>MGSETPQAEVGPTGCPHRSGPHSAKGSLEKGSPEDKEAKEPLWIRPDAPSRCTWQLGRPASESPHHHTAPAKSPKILPDILKKIGD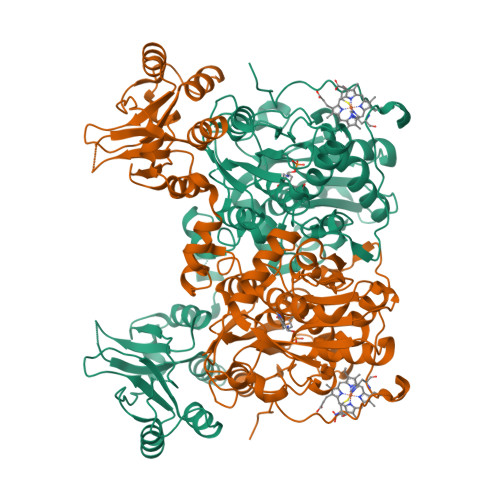TPMVRINKIGKKFGLKCELLAKCEFFNAGGSVKDRISLRMIEDAERDGTLKPGDTIIEPTSGNTGIGLALAAAVRGYRCIIVMPEKMSSEKVDVLRALGAEIVRTPTNARFDSPESHVGVAWRLKNEIPNSHILDQYRNASNPLAHYDTTADEILQQCDGKLDMLVASVGTGGTITGIARKLKEKCPGCRIIGVDPEGSILAEPEELNQTEQTTYEVEGIGYDFIPTVLDRTVVDKWFKSNDEEAFTFARMLIAQEGLLCGGSAGSTVAVAVKAAQELQEGQRCVVILPDSVRNYMTKFLSDRWMLQKGFLKEEDLTEKKPWWWHLRVQELGLSAPLTVLPTITCGHTIEILREKGFDQAPVVDEAGVILGMVTLGNMLSSLLAGKVQPSDQVGKVIYKQFKQIRLTDTLGRLSHILEMDHFALVVHEQQRQMVFGVVTAIDLLNFVAAQERDQKELHHHHHH[2x]> SSQIRQNYSTEVEAAVNRLVNLYLRAS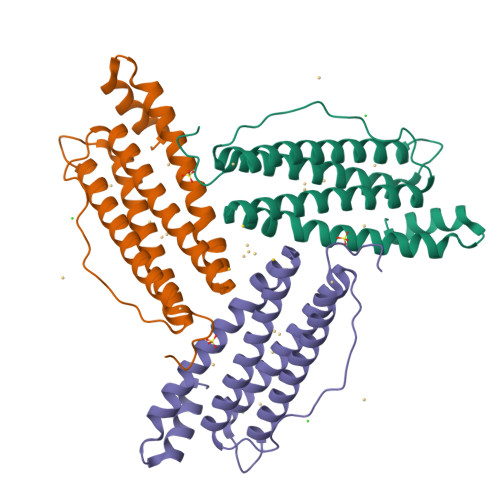YTYLSLGFYFDRDDVALEGVCHFFRELAEEKREGAERLLKMQNQRGGRALFQDLQKPSQDEWGTTLDAMKAAIVLEKSLNQALLDLHALGSAQADPHLCDFLESHFLDEEVKLIKKMGDHLTNIQRLVGSQAGLGEYLFERLTLKHD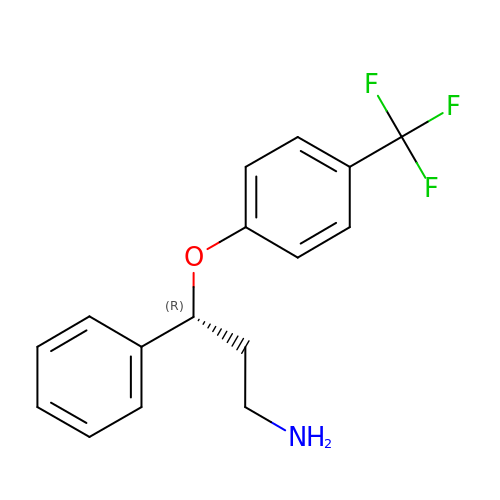(3R)-3-phenyl-3-[4-(trifluoromethyl)phenoxy]propan-1-amine | C16 H16 F3 N O | WIQRCHMSJFFONW-OAHLLOKOSA-N> 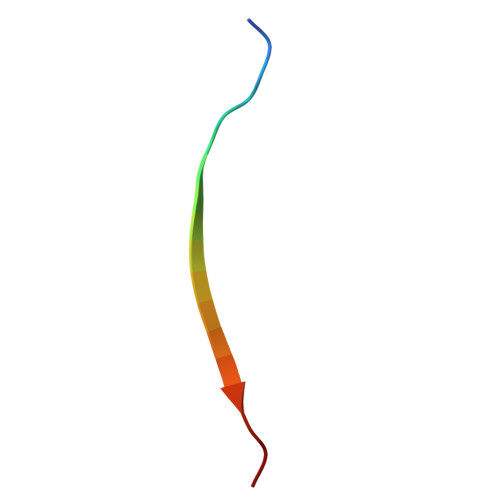PLEKASVVSKLFFSWTAP>[12x]FARSLSITTPEEMIEKAKGETAYLPCKFTLSPEDQGPLDIEWLISPADNQKVDQVIILYSGDKIYDDYYPDLKGRVHFTSNDLKSGDASINVTNLQLSDIGTYQCKVKKAPGVANKKIHLVVLV;>[12x]MRGSHHHHHHGSPPAAPITLWTGPGPSINGFINDTPVIRCFICLTRDSNLVTVNASFVGEGGYRIVSPTQSQFSLIMEFDQFGQLMSTGNINSTTTWGEKPWGNNTVQPRPSHTWKLCMPNREVYSTPAATISRCGLDSIAVDGAPSRSIDCMLIINKPKGVATYTLTFRFLNFNRLSGGTLFKTDVLTFTYVGENQ

To date, all Ads display a characteristic, icosahedral symmetry in which 240 subunits of the trimeric hexon protein form the facets and 12 copies of the penton, comprising the pentameric penton base protein and the externally projecting trimeric fiber, form the vertices. At least in vitro and for most cell types, the fiber mediates the initial attachment to primary receptors, such as the D1 domain of the coxsackievirus and adenovirus receptor (CAR), sialic acids, CD46, and others (for review see Zhang & Bergelson). Our results showing that the CAV-2 fiber head contains a sialic acid binding site creates a paradox: both HAd37 and CAV-2 fiber heads contain CAR and sialic acid binding sites - but HAd37 uses sialic acid and CD46, while CAV-2 uses CAR (CAV-2 does not use CD46 to infect cells, unpublished data) to infect cells. We show by structural analysis that the CAV-2 fiber head also contains a sialic acid binding site, but in contrast to HAd37 this site is modestly involved in hemagglutination.

To determine if sialic acid and CAR binding were mutually exclusive, we soaked CAV-2 or HAd37 fiber head crystals in complex with CAR in solutions containing sialyl-D-lactose. Crystals containing the complex with CAV-2 fiber head diffracted to 2.9 Å and contained 12 chains of fiber head bound to 12 chains of CAR D1 and 12 sialyl-D-lactose molecules in the asymmetric unit (space group I422). For both structures the electron density maps showed clear density for sialic acid, but not lactose, at the expected positions on the fiber heads. Our crystal structure of CAV-2 fiber head in complex with CAR and sialyl-D-lactose demonstrates that the ternary complex of the three molecules is stable. There is no indication that this should not be the case also in vivo. With respect to CAR affinity, the CAV-2 fiber head binds human CAR with the highest affinity of any fiber head known, which may favor its efficient hemagglutination. We cannot exclude the possibility that in some cell types sialic acid binding provides a first low-affinity attachment to the cell surface, while CAR-binding is followed in a second step, providing a high-affinity binding. Unexpectedly, we found that the CAV-2 fiber head harbors a sialic acid binding site.>[3x]MGSSHHHHHHLVPRGSHMMSRSDQENPFIFKSNRFQTLYENENGHIRLLQKFDKRSKIFENLQNYRLLEYKSKPHTLFLPQYTDADFILVVLSGKATLTVLKSNDRNSFNLERGDAIKLPAGTIAYLANRDDNEDLRVLDLAIPVNKPGQLQSFLLSGTQNQPSLLSGFSKNILEAAFNTNYE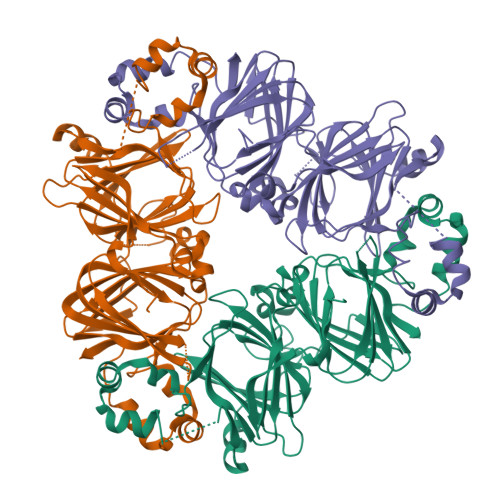EIEKVLLEQQEQEPQHRRSLKDRRQEINEENVIVKVSREQIEELSKNAKSSSKKSVSSESGPFNLRSRNPIYSNKFGKFFEITPEKNQQLQDLDIFVNSVDIKEGSLLLPNYNSRAIVIVTVTEGKGDFELVGQRNENQGKENDKEEEQEEETSKQVQLYRAKLSPGDVFVIPAGHPVAINASSDLNLIGFGINAENNERNFLAGEEDNVISQVERPVKELAFPGSSHEVDRLLKNQKQSYFANA> VEWTQQERSIIAGIFANLNYEDIGPKALARCLIVYPWTQRYFGAYGDLSTPDAIKGNAKIAAHGVKVLHGLDRAVKNMDNINEAYSELSVLHSDKLHVDPDNFRILGDCLTVVIAANLGDAFTVETQCAFQ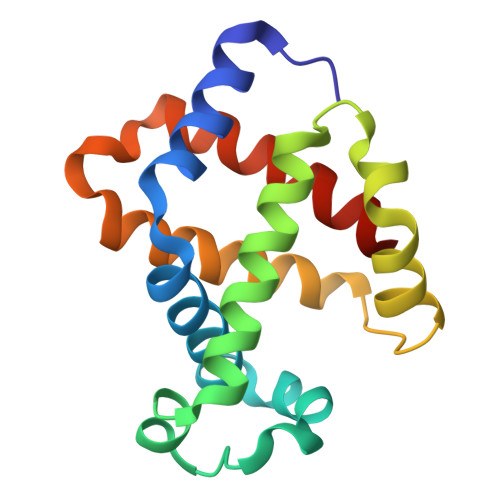KFLAVVVFALGRKYH> MRLLYLHADRFEYKTVKPALKNPPDPPGEASFGEALVVFTTVEDGDGPQTVMYAASDIASHSSRLKVTTVILYPYAHLSSRLAKPMAAHKRLIELEGALRTKFPGHVHRAPFGWYMSFSIACKGHPLAELSRSFTE

We have been interested in a D-aminoacyl-tRNA deacylase (DTD) fold that is present across the domains of life in two different functional contexts: as an N-terminal editing domain (NTD) of archaeal ThrRS, which specifically removes non-cognate L-serine mischarged on tRNAThr, and as a freestanding ‘chiral proofreading' enzyme, which removes D-amino acids from tRNAs in bacteria and eukaryotes. Both share a striking structural and mechanistic similarity highlighting a common ancestry. Here we show, with the help of structural, biochemical and biophysical studies from three distant organisms, that the substrate specificity in this domain is determined by a differential remodelling of the catalytic centre at the RNA–protein interface rather than just the presence or absence of catalytic water as previously proposed. While demonstrating that the tRNA provides the catalytic group, we show that the side chains within the recognition site are dispensable for the proofreading function, suggesting a primordial mode of protein- or peptide scaffold-based enzymatic activity evolved alongside that of RNA.

On the other hand, the Lys to Met mutant, although showed partial activity against L-Ser-(Ec)tRNAThr in our earlier work, in subsequent studies with not only PabNTD K121M but also the corresponding K116M and K122M mutants of ApNTD and MjNTD with multiple batches of protein showed a severely compromised activity, suggesting a crucial role of this residue in enzyme function. However, a direct role of Lys in catalysis is still highly unlikely considering that this position is naturally occupied by a Met in the structural homologue DTD. We solved the crystal structure of K121M mutant of PabNTD and K116M mutant of ApNTD with L-Ser3AA and L-Thr3AA to investigate the structural basis of the observed loss of activity. A significant repositioning of the crucial catalytic water was observed upon mutation of the polar Lys side chain to the non-polar Met side chain, which is present in DTD. This provides a clear structural basis for the loss of function in this mutant, despite its high binding affinity for the substrate. Therefore, we show that Lys plays a crucial role in positioning the water molecule for catalysis rather than acting as a nucleophile.> ATPNKTPPGADPKQLERTGTVREIGSQAVWSLSSCKPG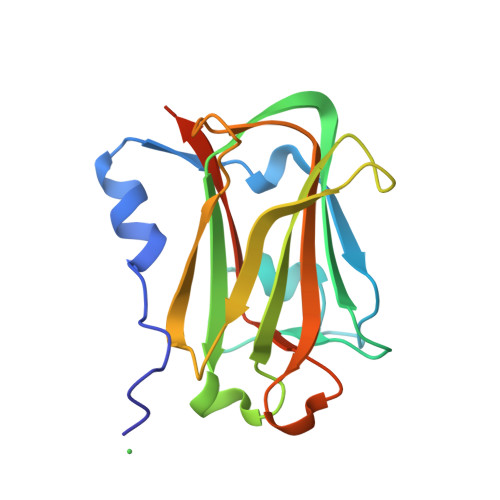FGVDQLRDDNLETYWQSDGSQPHLVNIQFRRKTTVKTLCIYADYKSDESYTPSKISVRVGNNFHNLQEIRQLELVEPSGWIHVPLTDNHKKPTRTFMIQIAVLANHQNGRDTHMRQIKIYTPVEESSIGKFPR>SNAMIRKYRYGAPFDTEALTEKIETAEEAFPYGEISQKEGFAFTYIMDEDDIVYGLGESNRGINKRGYCYISNCTDDPIHTEDKRSLYGAHNFIIVSGKTTFGLFFDYPSKLTFDIGYTRMDTLKVSCENADLDIYVIEGENAYDIVKQFRRVIGRSYIPPKFAFGFGQSRWGYTTKEDFRAVAKGYRENHIPIDMIYMDIDYMQDFKDFTVNEKNFPDFPEFVKEMKDQELRLIPIIDAGVKVEKGYEVYEEGVKNNYFCKREDGSDFVAAVWPGDTHFPDMLNPEARKWFGDKYRFLIDQGIEGFWNDMNEPAIFYSSEGLAEAKEFAGEFAKDTEGKIHPWAMQAKMKDIVNSPEDYKRFYHNVNGKKIRHDKVHNLFGYNMTRAAGEAFERIDPEKRFLMFSRSSYIGMHRYGGIWMGDNKSWWSHILLNLKMLPSLNMCGFMYTGADLGGFGDDTTRDLLLRFLALGVFTPLMRDHAAEGTREQECYQFENIEDFRSVINARYRLVPYLYSEYMKAALNDDMYFKPLGFVYPDDKMAIRVEDQLMLGNEIMIAPVY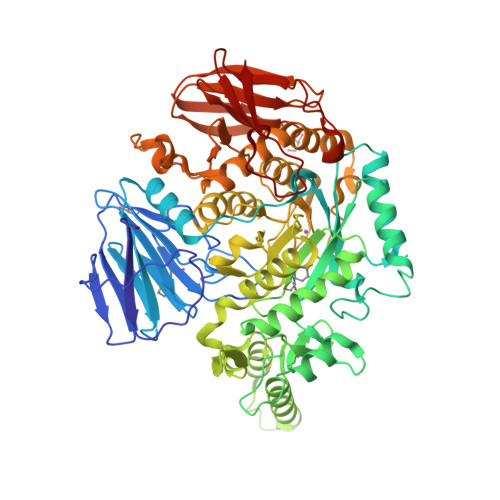EQNARGRYVYLPEEMKFIKFMPDGSISEEVLEKGVHYVDVALNEVPLFIRSGKCIPVAEAAECVKDIDTENMQLIGYEGSSYTLYEDDGIHKDYDKKENYRVLTK[2x]>[2x]SMRKSREYEHVRRDLDPNEVWEIVGELGDGAFGKVYKAKNKETGALAAAKVIETKSEEELEDYIVEIEILATCDHPYIVKLLGAYYHDGKLWIMIEFCPGGAVDAIMLELDRGLTEPQIQVVCRQMLEALNFLHSKRIIHRDLKAGNVLMTLEGDIRLADFGVSAKNLKTLQKRDSFIGTPYWMAPEVVMCETMKDTPYDYKADIWSLGITLIEMAQIEPPHHELNP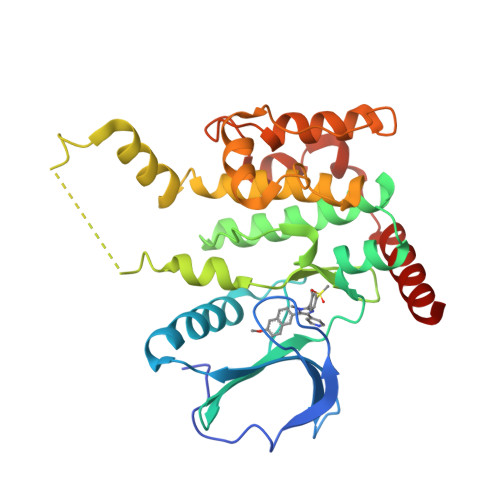MRVLLKIAKSDPPTLLTPSKWSVEFRDFLKIALDKNPETRPSAAQLLEHPFVSSITSNKALRELVAEAKAEVMEE> AGVGTVPMTDYGNDIEYYGQVTIGTPGKKFNLDFDTGSSDLWIASTLCTNCGSGQTKYDPNQSSTYQADGRTWSISYGDGSSASGILAKDNVNLGGLLIKGQTIELAKREAASFASGPNDGLLGLGFDTITTVRGVKTPMDNLISQGLISRPIFGVYLGKAKNGGGGEYIFGGYDSTKFKGSLTTVPIDNSRGWWGITVDRATVGTSTVASSFDGILDTGTTLLILPNNIAASVARAYGASDNGDGTYTISCDTSAFKPLVFSINGASFQVSPDSLVFEEFQGQCIAGFGYGNWGFAIIGDTFLK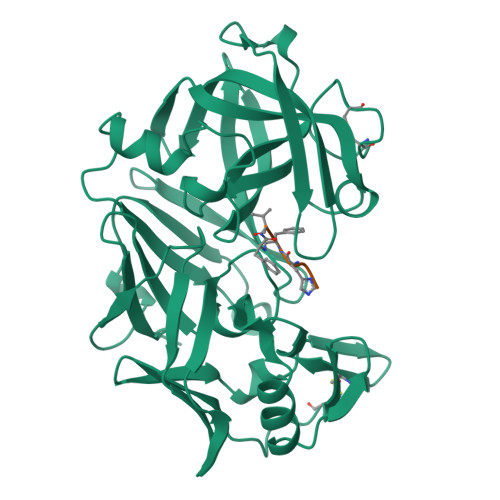NNYVVFNQGVPEVQIAPVAE;> HPFHXVY> GSTELTPDQQTLLHFIMDSYNKQRMPQEITNKILKEEFSAEENFLILTEMATNHVQVLVEFTKKLPGFQTLDHEDQIALLKG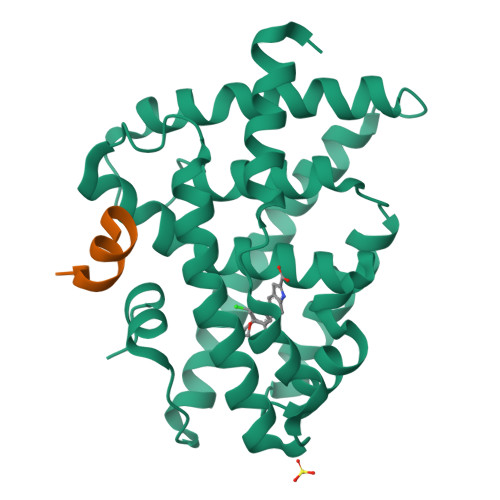SAVEAMFLRSAEIFNKKLPSGHSDLLEERIRNSGISDEYITPMFSFYKSIGELKMTQEEYALLTAIVILSPDRQYIKDREAVEKLQEPLLDVLQKLCKIHQPENPQHFACLLGRLTELRTFNHHHAEMLMSWRVNDHKFTPLLCEIWDVQ;> KESKDHQLLRYLLDKDEKDLR>[2x]MSPCGYYSKWRNRDRPEYRRNLRFRRFFSSIHPNAAAGSGFNGPGVFITSVTGVWLCFLCIFSMFVTAVVSVSPSSFYESLQVEPTQSEDITRSAHLGDGDEIREAIHKSQDAETKPTFYVCPPPTGSTIVRLEPPRTCPDYHLGKNFTEGIAVVYKENIAAYKFKATVYYKDVIVSTAGAGSSGTQITNRYADR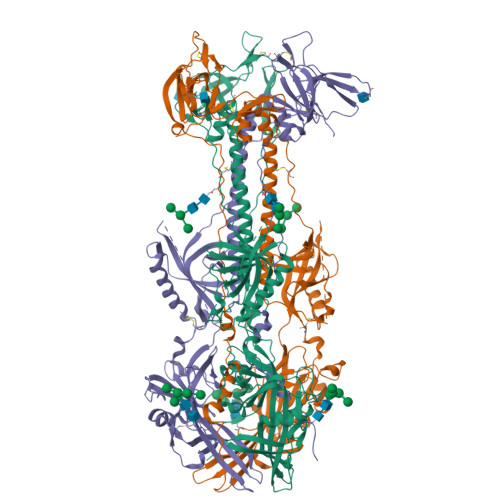VPIPVSEITDTIDKFGKCSSKATYVRNNHKVEAFNEDKNPQDMPLIASKYNSVGSKAWHTTNDTYMVAGTPGTYRTGTSVNCIIEEVEARSIFPYDSFGLSTGDIIYMSPFFGLRDGAYREHSNYAMDRFHQFEGYRQRDLDTRALLEPAARNFLVTPHLTVGWNWKPKRTEVCSLVKWREVEDVVRDEYAHNFRFTMKTLSTTFISETNEFNLNQIHLSQCVKEEARAIINRIYTTRYNSSHVRTGDIQTYLARGGFVVVFQPLLSNSLARLYLQELVRENTNHSPQKHPTRNTGSGGSVPVELRANRTITTTSSVEFAMLQFTYDHIQEHVNEMLARISSSWCQLQNRERALWSGLFPINPSALASTILDQRVKARILGDVISVSNCPELGSDTRIILQNSMRVSGSTTRCYSRPLISIVSLNGSGTVEGQLGTDNELIMSRDLLEPCVANHKRYFLFGHHYVYYEDYRYVREIAVHDVGMISTYVDLNLTLLKDREFMPLQVYTRDELRDTGLLDYSEIQRRNQMHSLRFYDIDKVVQGSHHHHHH> ATSDSNMLLNYVPVYVMLPLGVVNVDNVFEDPDGLKEQLLQLRAAGVDGVTVDVWWGIIELKGPKQYDWRAYRSLLQLVQECGLTLQAIMSFHQCGGNVGDIVNIPIPQWVLDIGESNHDIFYTNRSGTRNKEYLTVGVDNEPIFHGRTAIEIYSDYMKSFRENMSDFLESGLIIDIEVGLGPAGELRYPSYPQSQGWEFPGIGEFQCYDKYLKADFKAAVARAGHPEWELPDDAGKYNDVPESTGFFKSNGTYVTEKGKFFLTWYSNKLLNHGDQ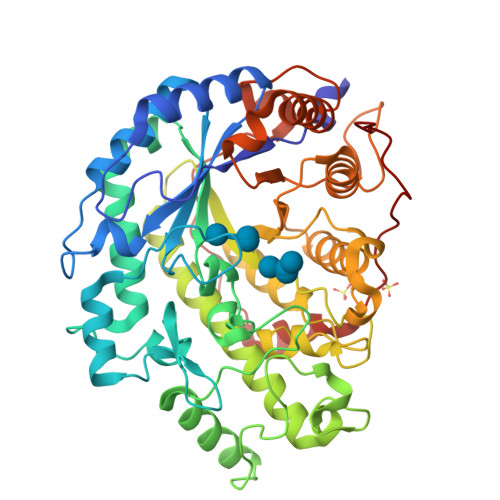ILDEANKAFLGCKVKLAIKVSGIHWWYKVENHAAELTAGYYNLNDRDGYRPIARMLSRHHAILNFTCLEMRDSEQPSDAKSGPQELVQQVLSGGWREDIRVAGENALPRYDATAYNQIILNARPQGVNNNGPPKLSMFGVTYLRLSDDLLQKSNFNIFKKFVLKMHADQDYCANPQKYNHAITPLKPSAPKIPIEVLLEATKPTLPFPWLPETDMKVDG> NGIVPDAGHQGPDVSAVNGGTQVINIVTPNNEGISHNQYQDFNVGKPGAVFNNALEAGQSQLAGHLNANSNLNGQAASLILNEVVSRNPSFLLGQAEVFGIAAEAVLSNPNGITCDGCGFINTSRSSLVVGNPLFENGQLKGY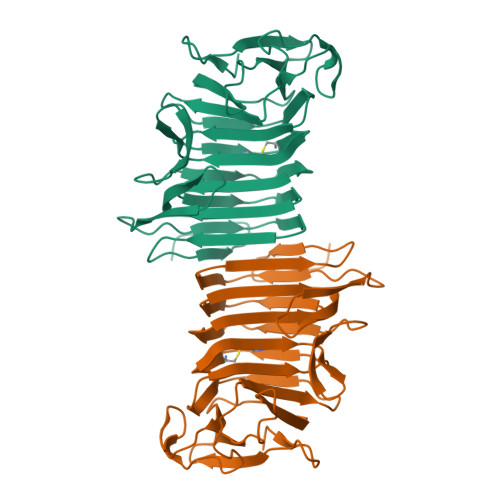STLNNTNLLSLGKNGLNTTGLLDLIAPRIDSRGKITAAEISAFTGQNTFSQHFDILSSQKPVSALDSYFFGSMQSGRIRIINTAEGSGVKLAGHHHHHH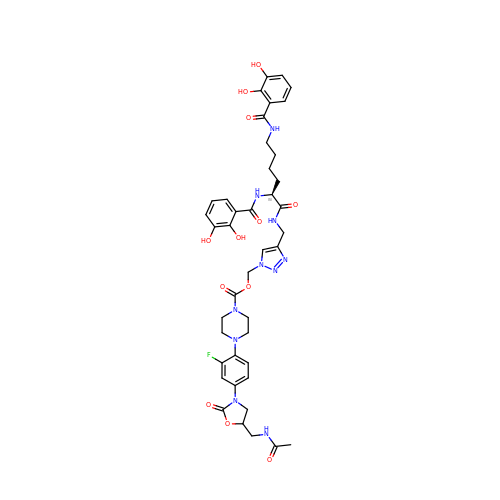BCV-L6 | C41 H47 F N10 O12 | AFDBLYUYBQJNFF-BDTAHNRFSA-N> MEFVMKQALGGATKDMGKMLGGD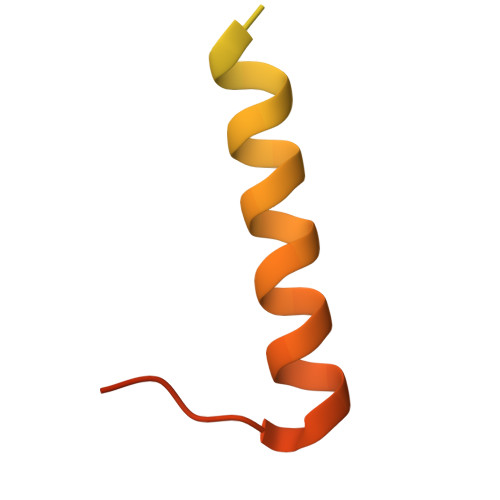EEKDPDAAKKEEERQEALRQAEEERKAKYAKMEAEREVMRQGIRDKYGIKKKEEREAEAQ3-amino-6-[4-(2-hydroxyethyl)phenyl]-N-[4-(morpholin-4-yl)pyridin-3-yl]pyrazine-2-carboxamide | C22 H24 N6 O3 | 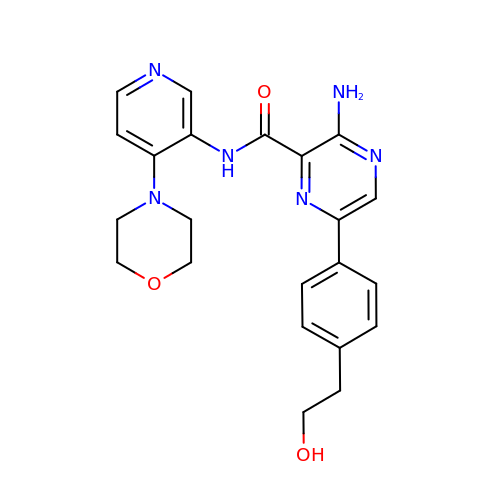UEECNVFACUZGKV-UHFFFAOYSA-N>SNADDLRDTVTRQIAPLMKQYAIPGMAIGIVADGKPYVFDYGVMSKQTGKPVTGDTLFEIGSVSKTLTATLASDAQEGGELSLADPAGKYLPELQGKPFGVVTLLQLGTHTPGGTPLQVPDSIRDDAGLIRYLDAWRPAYAPGTHRKYSNVAIGMLGWLTAKAMHQDFATLMEQRLFPAIGMTHTYINVPAARMADYAQGYTKDGKPVRMTEGMLWQPAYGVRTTAADLLRFVQANMGMIHTAPRLQRAIERTHTGYFRAGPLTQDLIWEQYPYPVALPTLLAGNAPKMLFDAVPASAIQPPLAPNPATWINKTGSTGGFSTY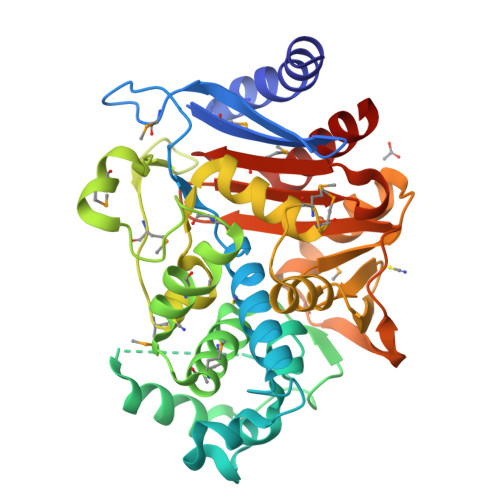VAFVPAKRIGIVMLANGNVPIEERVKAAYRILGSLGDA[2x]>MSVEKIPGYTYGETENRAPFNLEDLKLLKEAVMFTAEDEEYIQKAGEVLEDQVEEILDTWYGFVGSHPHLLYYFTSPDGTPNEKYLAAVRKRFSRWILDTSNRSYDQAWLDYQYEIGLRHHRTKKNQTDNVESVPNIGYRYAVAFIYPI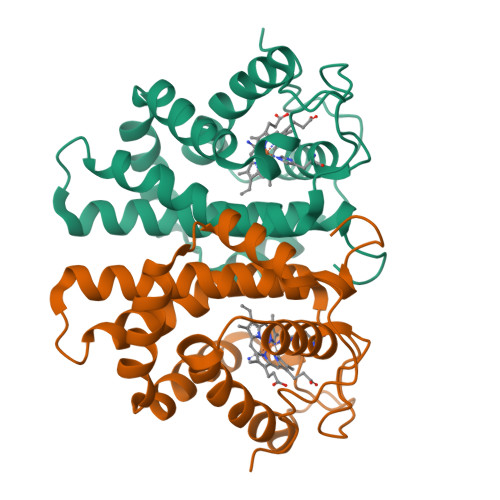TATMKPFLARKGHTPEEVEKMYQAWFKATTLQVALWSYPYVKYGDF[2x]(1R,5R)-5-{(1Z)-N-[(4'-fluorobiphenyl-4-yl)methoxy]butanimidoyl}-2,2-dimethyl-4,6-dioxocyclohexanecarbonitrile 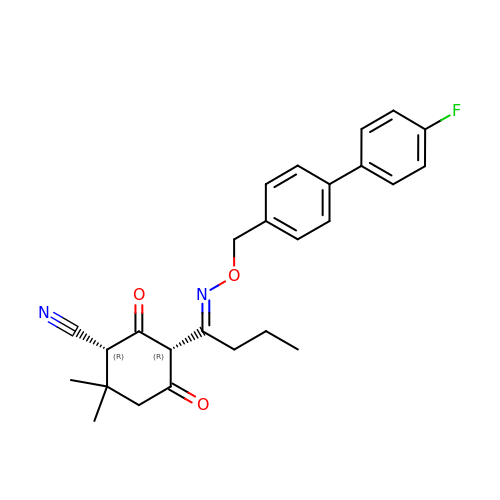| C26 H27 F N2 O3 | QRVDHQOKZPXAJH-FQRCLESUSA-N> SNAMLNTLIVGASGYAGAELVSYVNRHPHMTITALTVSAQSNDAGKLISDLHPQLKGIVDLPLQPMSDVRDFSADVDVVFLATAHEVSHDLAPQFLQAGCVVFDLSGAFRVNDRAFYEKYYGFTHQYPELLEQAVYGLAEWNVDKLNTANLIAVPGCYPTAAQLSLKPLIDGGLLDLTQWPVINATSGVSGAGRKAAISNSFCEVSLQPYGVFTHRHQPEIAVHLGAEVIFTPHLGNFPRGILETITCRLKAGVTHAQVADVLQKAYGDKPLVRLYDKGVPALKNVVGLPFCDIGFAVQGEHLIVVATEDNLLKGAAAQAVQCANIRFG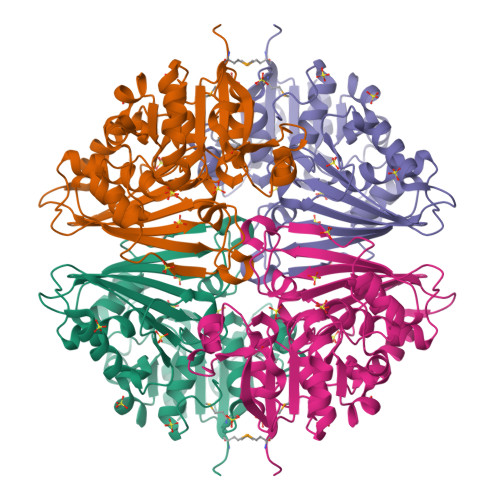FAETQSLI We earlier identified a putrescine transaminase spuC gene in Pseudomonas putida with preference to aliphatic diamines other than putrescine such as cadaverine and spermidine. A basic local alignment search tool (BLAST) analysis revealed a 76% protein sequence identity to a spuC gene from Pseudomonas aeruginosa, that was previously characterized to be part of a polyamine uptake and utilization pathway converting putrescine to 4-aminobutyraldehyde. In this study, we report on the detailed characterization (structural and biochemical) of the putrescine transaminase Pp-SpuC, and its application in the transamination of a comprehensive range of ketones/aldehydes for the production of a variety of benzylamine derivatives. We recognized the important dual substrate recognition of Pp-SpuC, accepting cadaverine or isopropylamine as the equilibrium shifting amine donor, and having excellent activity against a broad range of aromatic aldehyde derivatives bearing various electron-donating and electron-withdrawing substituents, as well as different heteroatoms in the ring, with excellent conversions.

A commercially available crystallogenesis screening set was employed, obtaining crystals under a number of different conditions after overnight incubation at 20°C. The best diffracting crystals were obtained in 0.2 M MgCl2, 0.1 M Bis-Tris pH 6.5, 25% PEG3350, then cryoprotected before freezing. There are two monomers in the asymmetric unit and the enzyme forms a tight dimer with predicted surface area of about 28710 Å2, with buried surface area of 3980 Å.2 Each monomer can be divided into two major domains. The large domain comprises residues 93–313 and folds into a sandwich of α/β/α comprising a core of seven stranded β-sheets with only β10 being antiparallel. The large domain is flanked by a small domain composed of two subdomains joined by a parallel β interaction between strand β3 and β14. The N-terminal subdomain forms extensive interactions with monomer 2 of the dimer which is important for active site formation, similar to what was observed with Cv-ωTA and Pse-ωTA. Unfortunately, all our attempts to obtain the structure of the complex of Pp-SpuC with PLP bound were unsuccessful. In the case of SpuC, the catalytic residue Lys289 is located on the loop between β4 and β10. Another disordered region of Pp-SpuC are amino acid residues 154–179 and 313–324. The homologous region 154–179 forms a “roof” above the cofactor binding site in the holo structure of Cv-ωTA, indicating its importance in PLP binding. The active key amino acid residues which constitute the small binding pocket and allow accommodation of substituents less bulky than an ethyl group are identified in Pp-SpuC as Phe23, Phe89′ (from the other subunit), Tyr154 and His155 (absent in the Pp-SpuC apo structure).

>MSTNNPQTREWQNLSGEHHLAPFSDYKQLKEKGPRIITKAQGVHLWDSEGHKILDGMAGLWCVAVGYGREELVQAAEKQMRELPYYNLFFQTAHPPALELAKAITDVAPEGMTHVFFTGSGSEGNDTVLRMVRHYWALKGKPHKQTIIGRINGYHGSTFAGACLGGMSGMHEQGGLPIPGIVHIPQPYWFGEGGDMTPDAFGIWAAEQLEKKILEVGEDNVAAFIAEPIQGAGGVIIPPETYWPKVKEILAKYDILFVADEVICGFGRTGEWFGSDYYDLKPDLMTIAKGLTSGYIPMGGVIVRDKVAKVISEGGDFNHGFTYSGHPVAAAVGLENLRILRDEQIVEKARTEAAPYLQKRLRELQDHPLVGEVRGLGMLGAIELVKDKATRSRYEGKGVGMICRTFCFENGLIMRAVGDTMIIAPPLVISHAEIDELVEKARKCLDLTLEAIRLE[2x]> MTWLPLNPIPLKDRVSMIFLQYGQIDVIDGAFVLIDKTGIRTHIPVGSVACIMLEPGTRVSHAAVRLAAQVGTLLVWVGEAGVRVYASGQPGGARSDKLLYQAKLALDEDLRLKVVRKMFELRFGEPAPARRSVEQLRGIEGSRVRATYALLAKQYGVTWNGRRYDPKDWEKGDTINQCISAATSCLYGVTEAAILAAGYAPAIGFVHTGKPLSFVYDIADIIKFDTVVPKAFEIARRNPGEPDREVRLA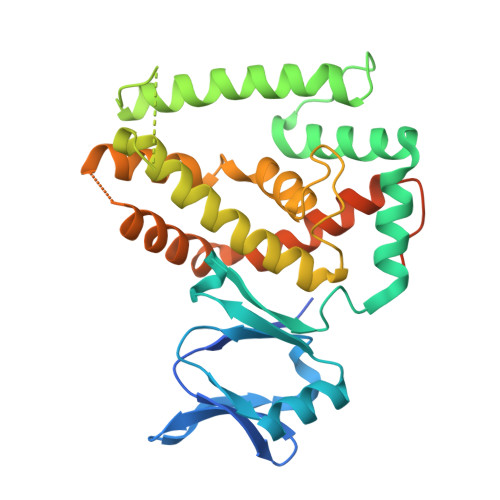CRDIFRSSKTLAKLIPLIEDVLAAGEIQPPAPPEDAQPVAIPLPVSLGDAGHRSS>[4x]MRGSHHHHHHGMASMRILLSNDDGVH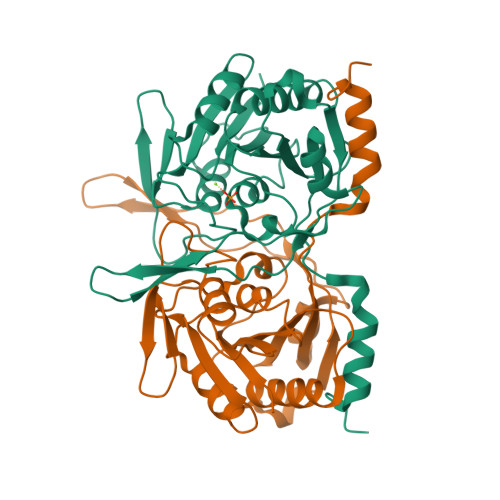APGIQTLAKALREFADVQVVAPDRNRSGASNSLTLESSLRTFTFDNGDIAVQMGTPTDCVYLGVNALMRPRPDIVVSGINAGPNLGDDVIYSGTVAAAMEGRHLGFPALAVSLNGYQHYDTAAAVTCALLRGLSREPLRTGRILNVNVPDLPLAQVKGIRVTRCGSRHPADKVIPQEDPRGNTLYWIGPPGDKYDAGPDTDFAAVDEGYVSVTPLHVDLTAHSAHDVVSDWLDSVGVGTQW>[2x]ENRAAQGDITAPGGARRLTGDQTAALRDSLSDKPAKNIILLIGDGMGDSEITAARNYAEGAGGFFKGIDALPLTGQYTHYALNK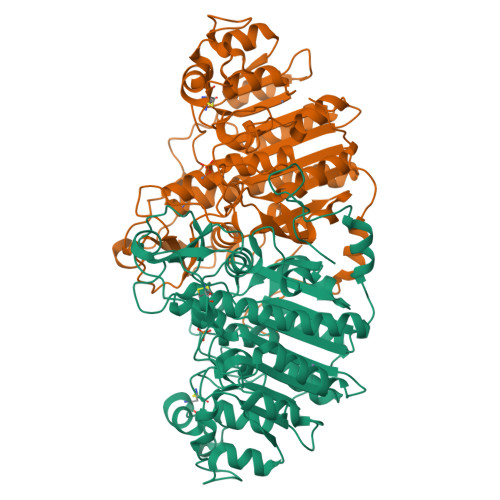KTGKPDYVTASAASATAWSTGVKTYNGALGVDIHEKDHPTILEMAKAAGLATGNVSTAELQAATPAALVAHVTSSKCYGPSATSEKCPGNALEKGGKGSITEQLLNARADVTLGGGAKTFAETATAGEWQGKTLREQAQARGYQLVSDAASLNSVTEANQQKPLLGLFADGNMPVRWLGPKATYHGNIDKPAVTCTPNPQRNDSVPTLAQMTDKAIELLSKNEKGFFLQVAGASIDAQDHAANPCGQIGETVDLDEAVQRALEFAKKEGNTLVIVTADHAHASQIVAPDTKAPGLTQALNTKDGAVMVMSYGNSEEDSQEHTGSQLRIAAYGPHAANVVGLTDQTDLFYTMKAALGLKWSHP>MAIGLPSINISFKELATTVKERSARGIIAMVLKDAKALGLNEIHEKEDIPVDLSAENKEYINLALMGNVNTPNKLLVYVIEGEADIQTALDFLETKEFNYLCMPKAVEADKTAIKNWIIKLRDIDKVKVKAVLGKVVGNHEGIINFTTEDVLVGEKKYSVDEFTSRVAGLIAGTPLSQSVTYTKLSDVVDIPKMTKVDAESRVNKGELILIKEAGAIRIARGVNSLTELTAEKGEMFQKIKIVDTLDIIHSDIRKVIIDDYIGKVTNSYDNKCLLIVAIKSYLEELEKSALIESDSTVEIDFEAQKSYLKSKGVDLSYMTLQEIKEANTGSKVFLKAKIKVLDAMEDIDLSIEI[18x];>MANMEARNVMSGTWGELWLDGNKVAEVKKFQAKMEFTKEDIIIAGQMGTDTKYMGYKGKGSITLYHVSSRMHKLIGEKIKRGSEPRFVAISKLNDPDSYGAERIAVKNIAFDDLTLADWEVGVKGEIEAPFTFTEYDFLDII[18x];>[6x]MLKYKEILETIIEILKKNFTESIFIDDESVQGSEGSCFFVSILSVICTP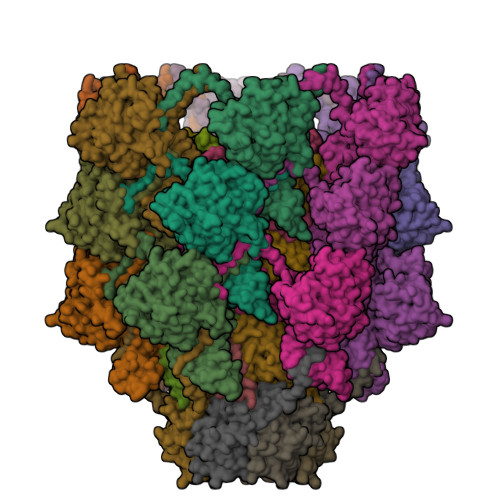VMLNTNNKDIVISIKYLPKPQSKSIRMYEISDELNKLFNRNIKVTDRKLNITKLEQSIKKEESIYVLNFTFTLNYLDSVYEEDVVYENMKEINLNLGE(4S)-4-[(E)-({3-hydroxy-2-methyl-5-[(E)-2-(1H-tetrazol-5-yl)ethenyl]pyridin-4-yl}methylidene)amino]-5-phenoxypentanoic 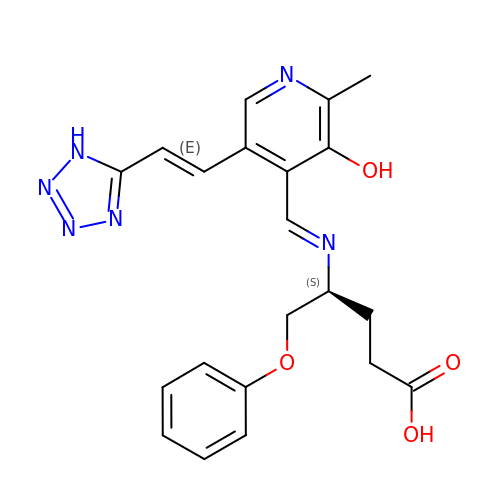acid | C21 H22 N6 O4 | QOYDXQUIAOTQIK-QFAAUBHJSA-N> MAAQGFLLIATFLLVLMVLARPLGSGLARLINDIPLPGTTGVERVLFRALGVSDREMNWKQYLCAILGLNMLGLAVLFFMLLGQHYLPLNPQQLPGLSWDLALNTAVSFVTNTNWQSYSGETTLSYFSQMAGLTVQNFLSAASGIAVIFALIRAFTRQSMSTLGNAWVDLLRITLWVLVPVALLIALFFIQQGALQNFLPYQAVNTVEGAQQLLPMGPVASQEAIKMLGTNGGGFFNANSSHPFENPTALTNFVQMLAIFLIPTALCFAFGEVMGDRRQGRMLLWAMSVIFVICVGVVMWAEVQGNPHLLALGTDSSINMEGKESRFGVLVSSLFAVVTTAASCGAVIAMHDSFTALGGMVPMWLMQIGEVVFGGVGSGLYGMMLFVLLAVFIAGLMIGRTPEYLGKKIDVREMKLTALAILVTPTLVLMGAALAMMTDAGRSAMLNPGPHGFSEVLYAVSSAANNNGSAFAGLSANSPFWNCLLAFCMFVGRFGVIIPVMAIAGSLVSKKSQAASSGTLPTHGPLFVGLLIGTVLLVGALTFIPALALGPVAEYLS;> MSRKQLALFEPTLVVQALKEAVKKLNPQAQWRNPVMFIVWIGSLLTTCISIAMASGAMPGNALFSAAISGWLWITVLFANFAEALAEGRSKAQANSLKGVKKTAFARKLREPKYGAAADKVPADQLRKGDIVLVEAGDIIPCDGEVIEGGASVDESAITGEAAPVIRESGGDFASVTGGTRILSDWLVIECSVNPGETFLDRMIAMVEGAQRRKTPNEIALTILLIALTIVFLLATATLWPFSAWGGNAVSVTVLVALLVCLIPTTIGGLLSAIGVAGMSRMLGANVIATSGRAVEAAGDVDVLLLDKTGTITLGNRQASEFIPAQGVDEKTLADAAQLASLADETPEGRSIVILAKQRFNLRERDVQSLHATFVPFTAQSRMSGINIDNRMIRKGSVDAIRRHVEANGGHFPTDVDQKVDQVARQGATPLVVVEGSRVLGVIALKDIVKGGIKERFAQLRKMGIKTVMITGDNRLTAAAIAAEAGVDDFLAEATPEAKLALIRQYQAEGRLVAMTGDGTNDAPALAQADVAVAMNSGTQAAKEAGNMVDLDSNPTKLIEVVHIGKQMLMTRGSLTTFSIANDVAKYFAIIPAAFAATYPQLNALNIMCLHSPDSAILSAVIFNALIIVFLIPLALKGVSYKPLTASAMLRRNLWIYGLGGLLVPFIGIKVIDLLLTVCGLV;> MSGLRPALSTFIFLLLITGGVYPLLTTVLGQWWFPWQANGSLIREGDTVRGSALIGQNFTGNGYFHGRPSATAEMPYNPQASGGSNLAVSNPELDKLIAARVAALRAANPDASASVPVELVTASASGLDNNITPQAAAWQIPRVAKARNLSVEQLTQLIAKYSQQPLVKYIGQPVVNIVELNLALDKLDE;> MSAGVITGVLLVFLLLGYLVYALINAE

KdpFABC is a high-affinity prokaryotic K+ uptake system that forms a functional chimera between a channel-like subunit (KdpA) and a P-type ATPase (KdpB). The heterotetrametric KdpFABC complex comprises four subunits, namely the channel-like KdpA, a member of the superfamily of K+ transporters (SKT), the P-type ATPase KdpB, the lipid-like stabilizer KdpF, and KdpC, whose function is still unknown. At high K+ levels, KdpFABC needs to be inhibited to prevent excessive K+ accumulation to the point of toxicity. This is achieved by a phosphorylation of the serine residue in the TGES162 motif in the A domain of the pump subunit KdpB (KdpBS162-P).

To determine the predominant states under turnover conditions, non-phosphorylatable KdpFABS162AC was incubated with 2 mM Mg2+-ATP and 50 mM KCl for 5 min at 24°C immediately before plunge freezing and analyzed by cryo-EM. The second structure obtained from the KdpFABS162AC sample under turnover conditions was resolved globally at 4.0 Å from ~28% of the initial particle set. In the respective cryo-EM map, a density is observable immediately adjacent to KdpBD307 and the TGES162 loop is in close proximity, which is the hallmark of an E2P or E2·Pi state. However, on closer inspection, the density fits better to a to a covalently bound phosphate than to a coordinated Pi. In light of the ambiguity at the given resolution, we have assigned this structure to an E2P state which might be transitioning to an E2·Pi. In comparison to the E1P·ADP state, the A domain in the E2P state has undergone a tilt of 60° and a rotation of 64° around the P domain, positioning the TGES162 loop to dephosphorylate KdpBD307 in the P domain, while the P domain is also tilted by 40°. (C, D) The outward-open half-channel closes off at the KdpA/KdpB interface, while a new, inward-open half-channel opens from the canonical substrate-binding site (CBS) in KdpB to the cytosol. The E1P·ADP and E2P structures obtained for KdpFABS162AC confirm that, in the absence of the inhibitory KdpBS162 phosphorylation, KdpFABC progresses through the entire Post-Albers cycle under turnover conditions, with the ADP release in the E1 state and the orthophosphate release in the E2 state likely being the rate-limiting steps that lead to an accumulation of the observed states.>[2x]MYIVNSNKSRGSSVERYIVSRLRDKGFAVIRAPASG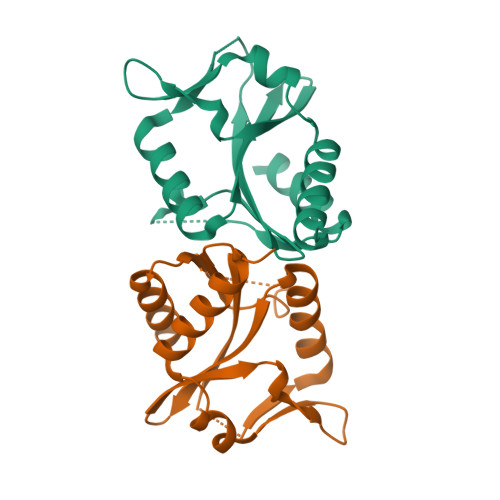SKRKDHVPDIIALKSGVIILIEVKSRKNGQKIYIEKEQAEGIREFAKRSGGELFLGVKLPKMLRFIKFDMLRQTEGGNYAIDLETVEKGMELEDLVRYVESKISRTLDSFL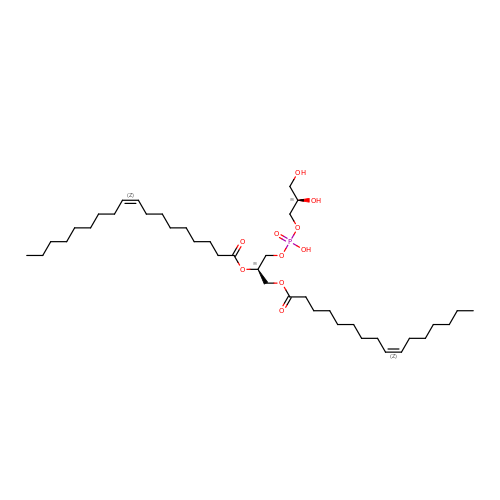(7Z,19R,22S,25R)-22,25,26-trihydroxy-16,22-dioxo-17,21,23-trioxa-22lambda~5~-phosphahexacos-7-en-19-yl (9Z)-octadec-9-enoate | C40 H75 O10 P | VCYYBLIRAQBPTM-CTDKCSBDSA-N> GPLGSMAASGLDHLKNGYRRRFCRPSRARDINTEQGQ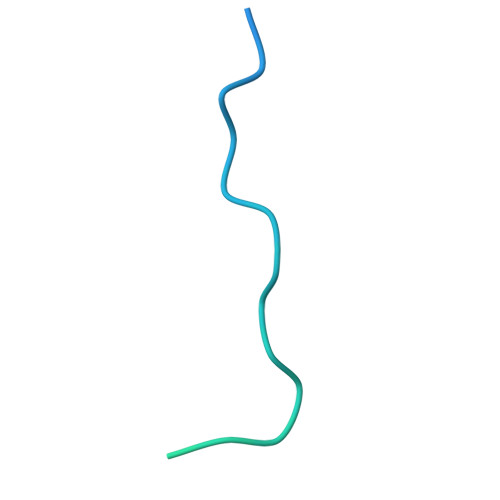NVLEILQDCFEEKSLANDFSTNSTKSVPNSTRKIKDTCI>MGSDKIHHHHHHMRYFSTDSPEVKTIVAQDSRLFQFIEIAGEVQLPTKPNPFQSLVSSIVEQQLSIKAASAIYGRVEQLVGGALEKPEQLYRVSDEALRQAGVSKRKIEYIRHVCEHVESGRLDFTELEGAEATTVIEKLTAIKGIGQWTAEMFMMFSLGRLDVLSVGDVGLQRGAKWLYGNGEGDGKKLLIYHGKAWAPYETVACLYLWKAAGTFAEEYRSLEELLHHGN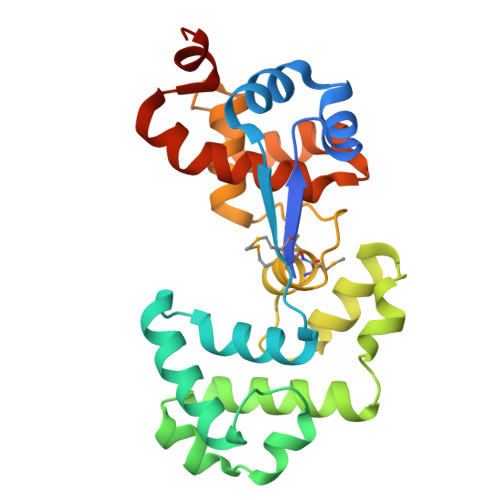QC[3x]> MDIIFYHPTFDTQWWIEALRKAIPQARVRAWKSGDNDSADYALVWHPPVEMLAGRDLKAVFALGAGVDSILSKLQAHPEMLNPSVPLFRLEDTGMGEQMQEYAVSQVLHWFRRFDDYRIQQNSSHWQPLPEYHREDFTIGILGAGVLGSKVAQSLQTWRFPLRCWSRTRKSWPGVQSFAGREELSAFLSQCRVLINLLPNTPETVGIINQQLLEKLPDGAYLLNLARGVHVVEDDLLAALDSGKVKGAMLDVF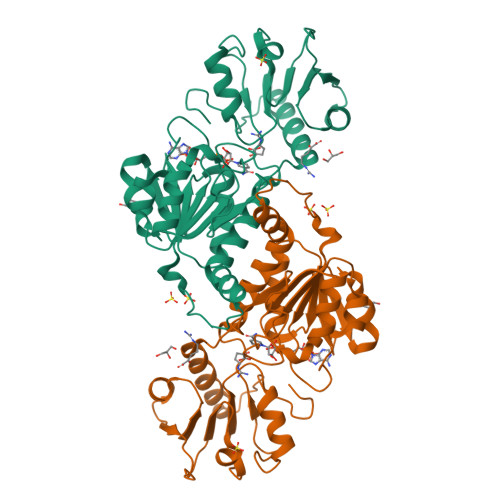NREPLPPESPLWQHPRVTITPHVAAITRPAEAVEYISRTIAQLEKGEKVCGQVDRARGY> SNAMQRYLWQQADGKRHVYDTARHRVQAGRPFTALCGETVTPQTERGDLTAGLWFDG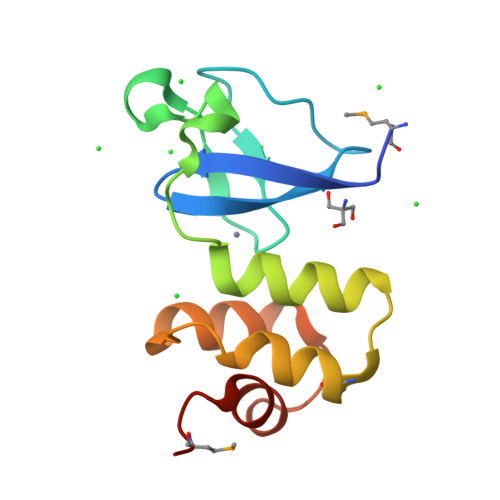ECPVCTIALAKALGWPMREISDLAHRFDWSPALITRLAEVLHCSFGEVVELTGARMVDA>[2x]MEFTEFNLNELIREVYVLFEEKIRKMNIDFCFETDNEDLRVEADRTRIKQVLINLVQNAIEATGENGKIKI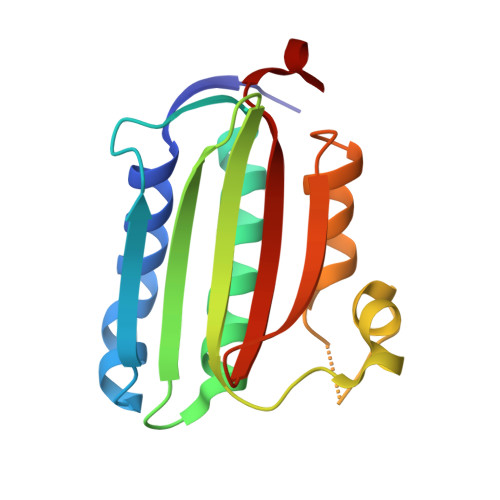TSEDMYTKVRVSVWNSGPPIPEELKEKIFSPFFTTKTQGTGLGLSICRKIIEDEHGGKIWTENRENGVVFIFEIPKTPEKR> NNDDPVENFVESTLKEVLVVPDTKPSGPQHTTKPSILGAMEIGASSNATPESTIETRYVYNTNTNAEADVEMFLGRSALWGKVTLTRQYAKWEINFQEQAHIRKKFEFFTYLRFDMEVTIVTNNKGLMQIMFVPPGIDHPETHDDRKWDSASNPSVFFQPKSGFPRFTIPFTGLASAYYMFYDGYDKPKGSDNNEYGIAPTNDMGLLCFRTLDNSGGNDVKIYVKPKHITAWVPRPPRATQYTHKYSTNYHYKPNSSGPDEHVLKDRHFIKTRPLISSA;> GLPTRLPSGSQQFMTTEDEQSPNILPGFHPSKKIHIPGMITNVMHMARVDSFIPINNIQGEVGKVSMYYITVTKKTVTERILVLPLEMSNTLFATTLLGEVLNYYANWSGSITITFMCVCDAFSTGKFLVAYTPPGGKLPEDRKQAMLGVHIIWDLGLQSSCTIVVPWISSGFYRRTKADSFTHGGYVSLWYQTAFVPPVSGGTGSILATCSACPDMSVRMLRDSPMMEQKNELQ;> SPSVEACGYSDRLKQITIGNSTITTQDSLHTVLAYGEWPTYLSDIDATSVDKPTHPETSADRFYTLDSVEWQVGSHGWWWKLPDALKDMGVFGQNMYYHSMGRSGFIIHTQCNATKFHSGALIVAVIPEHQLAYVGGVKVNVGYDHTHPGQSGHQIRGPSQSNDRSGGKPDEDPLFNCNGTLLGNITIFPHQIINLRTNNSSTIVVPYINCVPMDNMLKHNNLSLVIIPLVPLRPGSSGINSVPITVTIAPYKSEFSGAMEAQRQ;> GAQVSRQNNGTHENGVTASNGSVIKYFNINYYKDSASSGLSRQDFSQDPSKFTQPLVDTLTN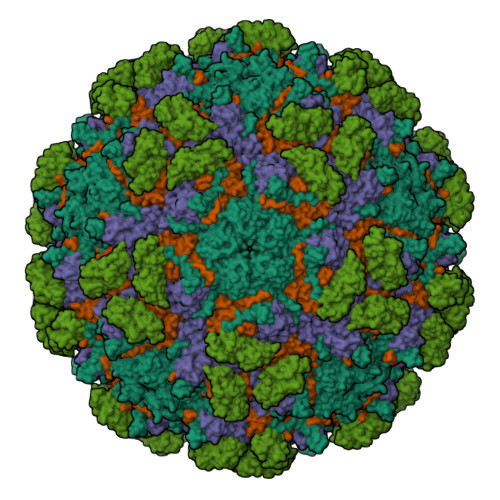PALM;> MASDYKDDDDKLHLILLPATGNVAENSPPGTSVHKFSVKLSASLSPVIPGFPQIVNSNPLTEAFRVNWLSGTYFEVVTTGMEQLDFETGPNIFDLQIYVKDEVGVTDLQVLTVQVTDVNEPPQFQGNLAEGLHLYIVERANPGFIYQVEAFDPEDTSRNIPLSYFLISPPKSFRMSANGTLFSTTELDFEAGHRSFHLIVEVRDSGGLKASTELQVNIVNLNDEVPRFTGGTKHHHHHH> SMKTDNAMKKIKLAIDGINQAIDNFNEVQTFTTINQLNHFKEKLMNCEHLIQLN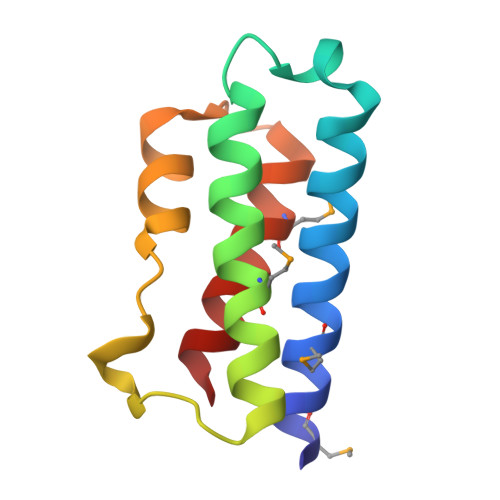NIPDKSHRNLGISRIIIDQWPFDSELGCMIINAESEYKSL> KAGSAAAPFTESLNRVIATVGTVSISELDLDDATEKYNRLQKHLKHEDYRKSFRTRIIDFLIDRAIVDVVAEEESIQVNEQRVDSEIEKRMEVMGITNRKQFEKTMETSSGMPFELWVTELPYQIKKGQLLQLKIAVPPPNEQEIRSWYNQNKDKVGFEIRYRIISIAPENDSIQEENRLYKEVSEIRKSILADPSSFALIAGSPRNDPALRARRGMVEWISSFDLYKYSKITATIAAPLPNGGVSEVFRDERKRYCILKIEGKRPTPMENLRGGIQNILYRDKEEDTFHR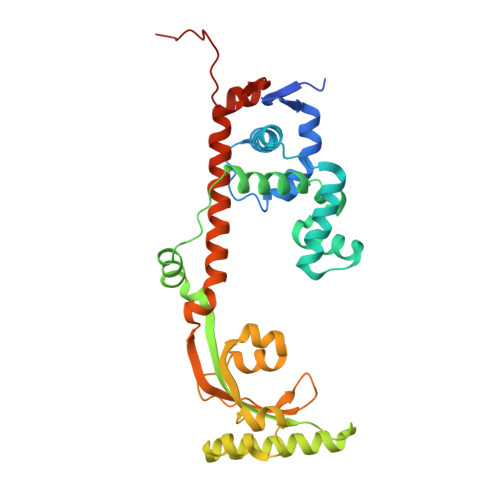WLKESRAEIPIQIFDEAYRKENKIPLKEETFHLD> MDPSSRDSQRNLLVIALLFVSFMIWQAWEQDKNPQPQAQQTTQTTTTAAGSAADQGVPASGQGKLISVKTDVLDLTINTRGGDVEQALLPAYPKELNSTQPFQLLETSPQFIYQAQSGLTGRDGPDNPANGPRPLYNVEKDAYVLAEGQNELQVPMTYTDAAGNTFTKTFVLKRGDYAVNVNYNVQNAGEKPLEISSFGQLKQSITLPPHLDTGSSNFALHTFRGAAYSTPDAAYAAYAFDTIADNENLNISSKGGWVAMLQQYFATAWIPHNDGTNNFYTANLGNGIAAIGYKSQPVLVQPGQTGAMNSTLWVGPEIQDKMAAVAPHLDLTVDYGWLWFISQPLFKLLKWIHSFVGNWGFSIIIITFIVRGIMYPLTKAQYTSMAKMRMLQPKIQAMRERLGDDKQRISQEMMALYKAEKVNPLGGCFPLLIQMPIFLALYYMLMGSVELRQAPFALWIHDLSAQDPYYILPILMGVTMFFIQKMSPTTVTDPMQQKIMTFMPVIFTVFFLWFPSGLVLYYIVSNLVTIIQQQLIYRGLEKRGLHSREKKKSHHHHHH;> MHHHHHHMLNRYPLWKYVMLIVVIVIGLLYALPNLFGEDPAVQITGARGVAASEQTLIQVQKTLQEEKITAKSVALEEGAILARFDSTDTQLRAREALMGVMGDKYVVALNLAPATPRWLAAIHAEPMKLGLDLRGGVHFLMEVDMDTVLGKLQEQNIDSLRSDLREKGIPYTTVRKENNYGLSITFRDAKARDEAIAYLSKRHPDLVISSQGSNQLRAVMSDARLSEAREYAVQQNINILRNRVNQLGVAEPVVQRQGADRIVVELPGIQDTARAKEILGATATLEFRLVNTNVDQAAAASGRVPGDSEVKQTREGQPVVLYKRVILTGDHITDSTSSQDEYNQPQVNISLDSAGGNIMSNFTKDNIGKPMATLFVEYKDSGKKDANGRAVLVKQEEVINIANIQSRLGNSFRITGINNPNEARQLSLLLRAGALIAPIQIVEERTIGPTLGMQNIEQGLEACLAGLLVSILFMIIFYKKFGLIATSALIANLILIVGIMSLLPGATLSMPGIAGIVLTLAVAVDANVLINERIKEELSNGRTVQQAIDEGYRGAFSSIFDANITTLIKVIILYAVGTGAIKGFAITTGIGVATSMFTAIVGTRAIVNLLYGGKRVKKLSI;> MHHHHHHDDDDKAMGANTEAQGSGRGLEAMKWVVVVALLLVAIVGNYLYRDIMLPLRALAVVILIAAAGGVALLTTKGKATVAFAREARTEVRKVIWPTRQETLHTTLIVAAVTAVMSLILWGLDGILVRLVSFITGLRF;> MAQEYTVEQLNHGRKVYDFMRWDYWAFGISGLLLIAAIVIMGVRGFNWGLDFTGGTVIEITLEKPAEIDVMRDALQKAGFEEPMLQNFGSSHDIMVRMPPAEGETGGQVLGSQVLKVINESTNQNAAVKRIEFVGPSVGADLAQTGAMALMAALLSILVYVGFRFEWRLAAGVVIALAHDVIITLGILSLFHIEIDLTIVASLMSVIGYSLNDSIVVSDRIRENFRKIRRGTPYEIFNVSLTQTLHRTLITSGTTLMVILMLYLFGGPVLEGFSLTMLIGVSIGTASSIYVASALALKL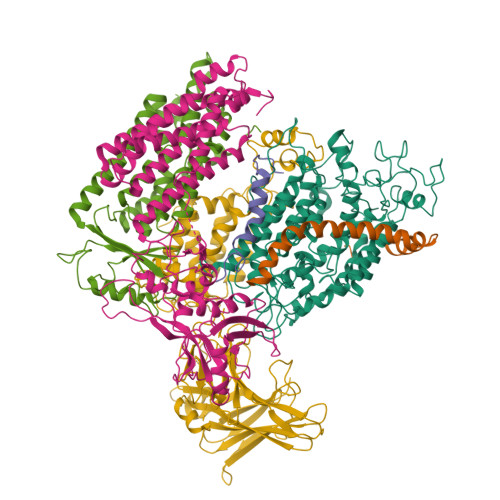GMKREHMLQQKVEKEGADQPSILP;> VGTGWYSGSPGILYHWPEVLRIQELIMYEALLVVFLIVAIGLVGLIMLQQGKGADMGASFGAGASATLFGSSGSGNFMTRMTALLATLFFIISLVLGNINSNKTNKGSEWENLSAPAKTEQTQPAAPAKPTSDIPN;> VWNCERITISHRKQTMAKQPGLDFQSAKGGLGELKRRLLFVIGALIVFRIGSFIPIPGIDAAVLAKLLEQQRGTIIEMFNMFSGGALSRASIFALGIMPYISASIIIQLLTVVHPTLAEIKKEGESGRRKISQYTRYGTLVLAIFQSIGIATGLPNMPGMQGLVINPGFAFYFTAVVSLVTGTMFLMWLGEQITERGIGNGISIIIFAGIVAGLPPAIAHTIEQARQGDLHFLVLLLVAVLVFAVTFFVVFVERGQRRIVVNYAKRQQGRRVYAAQSTHLPLKVNMAGVIPAIFASSIILFPATIASWFGGGTGWNWLTTISLYLQPGQPLYVLLYASAIIFFCFFYTALVFNPRETADNLKKSGAFVPGIRPGEQTAKYIDKVMTRLTLVGALYITFICLIPEFMRDAMKVPFYFGGTSLLIVVVVIMDFMAQVQTLMMSSQYESALKKANLKGYGR>MPKYNLRIGNRRVPIASTDTPLSEAIGKRLASSTPQTNVDSMGGGHSYQFNGQDLTFEDLRDIKDVRDSGGQVAQLMDYKALLNFGEGCEIHVEGDDETKQLVDGEPMTLSEWLEDAFPHLDLLVLDLGGDALWYPYAVGEIQETITGEFKEALPAEPWTLMPESDAQGKVQAWHQRTKTHGGYQTQTLPADDLWHIVINKASARDEVGISEVLRNKDEIQAFKQNEAAINQAIELHGFPQRHVKVGKEDGAPVRDNDLRRVRTIFDPRTTDANTAYFTGQDVDVETLEAHNFDYSAIHEMDMRNLTTALGLPLEAGNVGADGLGSGKPAELRFALLKLAIKANQRSFSVQFVERVMRPVVRDYSPFDHEADIRLEINDPLEDIGEVADLIQQVGDYMTNEQVAEKLDLPAPEDDEVADSYRSPADMEKDEAGVQDEPFGGMFAGRDMGNRCLGEGITDDELQHAPEWDRPLLEMYQGVTNPESDTSRTLVSFSSSGTPEFVLERIRESIMDGALFSEFDNIPSSRLMELRQTFADELGTDNFTLDSITDALMDFEADLTRDAAERIARTESSAVLNHAREISYEERGEGNELFYWTGADLGDSRQTEACAWLIRQTNPFSGGTPVPMNELRDMVDEAPSHDDSMDNNLARPDSWVVHPNERSSFVKAPPNWEQL[12x];>MPDPSIDEVSKSDWDALTTQEQDDIISQVENLSSTGWVNTSRERKAEAIRSAIAERDTLYSGNMSRLPTLDGDAEYFTLYLSAHKIQLFEGGEAQSESGEGGSVSYSTGGGGEKDLQKTRYGRMALEYVWEDNSIAALRTY[12x]

Here, we present the near-atomic resolution structure of Haloferax tailed virus 1 (HFTV1), an archaeal virus thriving in extreme salinity. Through single-particle analysis, we obtained near-atomic resolution maps of DNA-filled and empty virions, enabling us to assemble full atomic models of the virus pre- and post-DNA release, including all structural protein components. The full atomic structure revealed that the virus has a length of 1350 Å and an icosahedral head with a diameter of ~600 Å. The tail has a length of 560 Å and terminates into a baseplate with three radiating TFs of ~190 Å in length.

During image processing, we noticed that the sample contained DNA-filled particles as well as those that had already ejected their DNA genomes. The empty structure corresponds to a postinfection state. (C) Cross section of the empty virus, where the dsDNA, tape measure protein, baseplate hub and tail fibers are missing. Instead, a plug-like density appears to cap the portal protein. Comparing the portal structures of the DNA-filled and empty capsid shows that the latter has a plug-like density, which is missing in the former. The structure of the PP itself does not show substantial differences between the two states, indicating that large scale conformational changes in this protein are not required to facilitate DNA release. Moreover, the heads of filled and empty viruses show no notable differences, indicating that DNA release does not lead to any structural changes in the head.2-chloro-N-{2-[(5-chloro-2-{[4-(4-methylpiperazin-1-yl)phenyl]amino}pyrimidin-4-yl)oxy]phenyl}acetamide 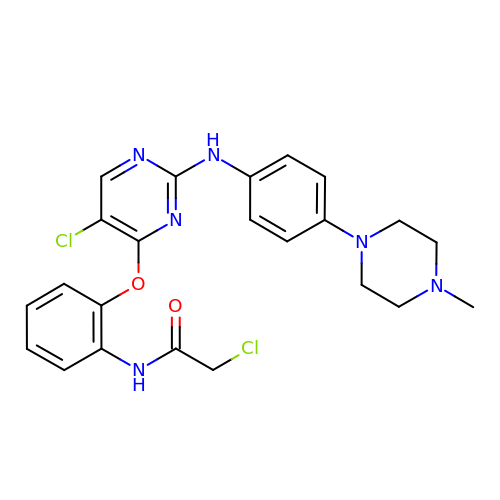| C23 H24 Cl2 N6 O2 | NQUKOQARFOAHTI-UHFFFAOYSA-N> WSHPQFEKVPIKYLPEENVHDADFGEQKDISEINLAAGLDLFQGDILLQKSRNGLRDPNTRWTFPIPYILADNLGLNAKGAILYAFEMFRLKSCVDFKPYEGESSYIIFQQFDGCWSEVGDQHVGQNISIGQGCAYKAIIEHEILHALGFYHEQSRTDRDDYVNIWWDQILSGYQHNFDTYDDSLITDLNTPYDYESLMHYQPFSFNKNASVPTITAKIPEFNSIIGQRLDFSAIDLERLNRMYNCTTTHTLLDHCTFEKANICGMIQGTRDDTDWAHQDSAQAGEVDHTLLGQCTGAGYFMQFSTSSGSAEEAALLESRILYPKRKQQCLQFFYKMTGSPSDRLVVWVRRDDSTGNVRKLVKVQTFQGDDDHNWKIAHVVLKEEQKFRYLFQGTKGDPQNSTGGIYLDDITLTETPCPTGVWTVRNFSQVLENTSKGDKLQSPRFYNSEGYGFGVTLYPNSRESSGYLRLAFHVCSGENDAILEWPVENRQVIITILDQEPDVRNRMSSSMVFTTSKSHTSPAINDTVIWDRPSRVGTYHTDCNCFRSIDLGWSGFISHQMLKRRSFLKNDDLIIFVDFEDITHLS

The zinc-dependent metalloprotease meprin α is predominantly expressed in the brush border membrane of proximal tubules in the kidney and enterocytes in the small intestine and colon. In normal tissue homeostasis meprin α performs key roles in inflammation, immunity, and extracellular matrix remodelling. In contrast to meprin β, meprin α is secreted into the extracellular space, whereupon it oligomerises to form giant assemblies and is the largest extracellular protease identified to date (~6 MDa). Here, using cryo-electron microscopy, we determine the high-resolution structure of the zymogen and mature form of meprin α, as well as the structure of the active form in complex with a prototype small molecule inhibitor and human fetuin-B. Our data reveal that meprin α forms a giant, flexible, left-handed helical assembly of roughly 22 nm in diameter.

The zymogen form of meprin α is plugged by an α-helical pro-peptide that sterically occludes the active site. The pro-peptide forms a small helical cork which plugs the active core and thus sterically occludes the active site. Cleavage of an exposed flexible loop, defined by residues L61-L67 located distal to the active site, releases the pro-peptide and exposes the catalytic core of the active site. Accordingly, the steric occlusion of the active site represents the major autoinhibitory mechanism. Secondly, the zymogen is converted to the active state by proteolytic removal of the pro-peptide. Comparison between the cryo-EM reconstructions of the latent and activated states reveal subtle conformational changes about the M12A catalytic domain. The subunit is a compact triad comprising the globular M12A protease, MAM and MATH domains. The meprin α M12A domain is typical, containing the catalytic zinc ion within the active site.(2S)-2-[(Z)-3-[2-(diethylamino)ethyl-[[4-[4-(trifluoromethyl)phenyl]phenyl]methyl]amino]-1-oxidanyl-3-oxidanylidene-prop-1-enyl]pyrrolidine-1-carboxylic acid 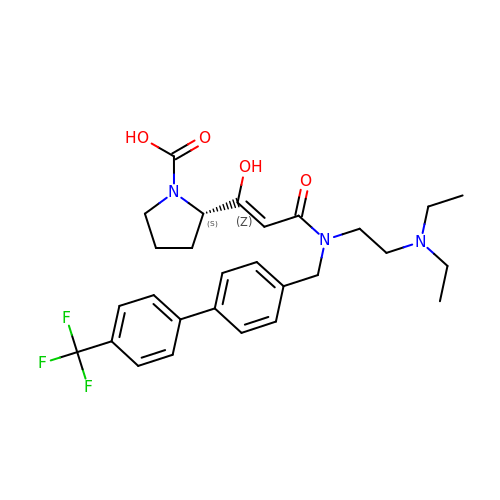| C28 H34 F3 N3 O4 | GTFYUFYLBSPPRI-BUFPPZMGSA-N> V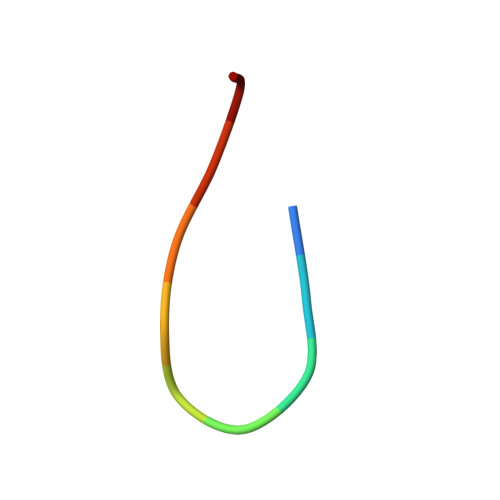AQGGAAGLA>DRLKGKVAIVTGGTLGIGLAIADKFVEEGAKVVITGRHADVGEKAAKSIGGTDVIRFVQHDASDEAGWTKLFDTTEEAFGPVTTVVNNAGIAVSKSVEDTTTEEWRKLLSVNLDGVFFGTRLGIQRMKNKGLGASIINMSSIEGLVGDPTQGAYNASKGAVRIMSKSAALDCALKDYDVRVNT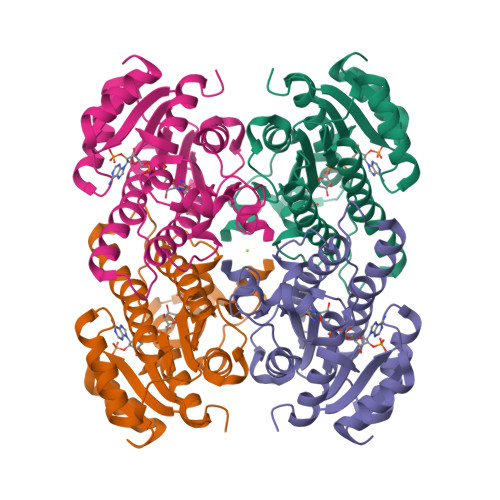VHPGPIKTPLVDDLEGAEEMMSQRTKTPMGHIGEPNDIAWICVYLASDESKFATGAEFVVDGGYTAQ[4x]>[2x]SNARIMEEKALEVYDLIRTIRDPEKPNTLEELEVVSESCVEVQEINEEEYLVIIRFTPTVPHCSLA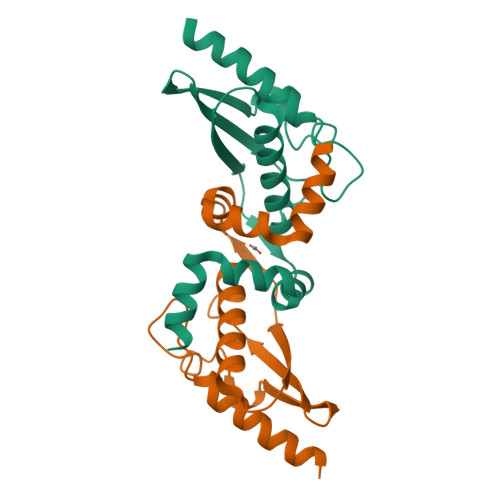TLIGLCLRVKLQRCLPFKHKLEIYISEGTHSTEEDINKQINDKERVAAAMENPNLREIVEQCVL> SQ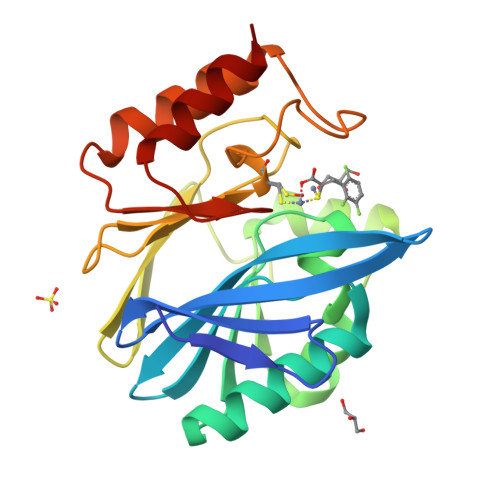KVEKTVIKNETGTISISQLNKNVWVHTELGSFNGEAVPSNGLVLNTSKGLVLVDSSWDDKLTKELIEMVEKKFQKRVTDVIITHAHADRIGGIKTLKERGIKAHSTALTAELAKKNGYEEPLGDLQTVTNLKFGNMKVETFYPGKGHTEDNIVVWLPQYNILVGGCLVKSTSAKDLGNVADAYVNEWSTSIENVLKRYRNINAVVPGHGEVGDKGLLLHTLDLLK>[4x]SAPADYFRILVQQFEVQLQQYRQQIEELENHLATQANNSHITPQDLSMAMQKIYQTFVALAAQLQSIHENVKVLKEQYLGYRKMFLGDA;>SYYIDADLLREIKQHLKQQQE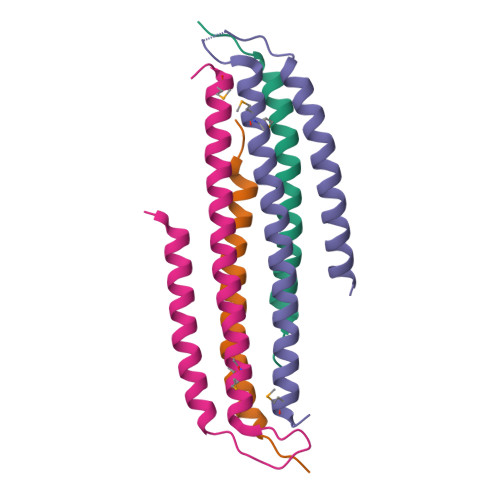GLSHLISIIKDDLEDIKLV[4x]4-[4-chloranyl-2-(1~{H}-pyrazol-4-yl)phenoxy]-3-cyano-~{N}-(1,3-thiazol-2-yl)benzenesulfonamide 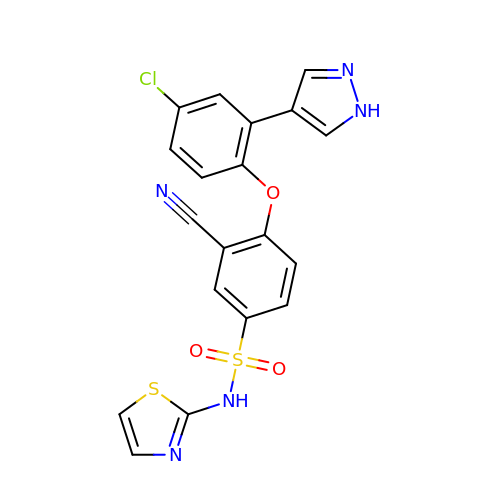| C19 H12 Cl N5 O3 S2 | XPZRWGQUAVWXIG-UHFFFAOYSA-N4-({4-[(3R)-3-amino-4-(2,4,5-trifluorophenyl)butanoyl]-1,4-diazepan-1-yl}carbonyl)benzoic 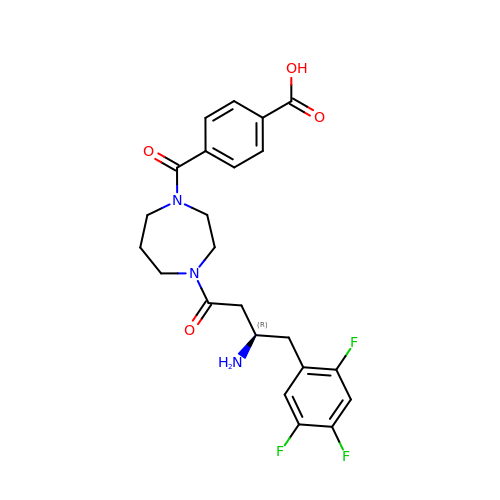acid | C23 H24 F3 N3 O4 | NXUBRAZWHJADLI-QGZVFWFLSA-N>MKTENAKTNQTLVENSLNTQLSNWFLLYSKLHRFHWYVKGPHFFTLHEKFEELYDHAAETVD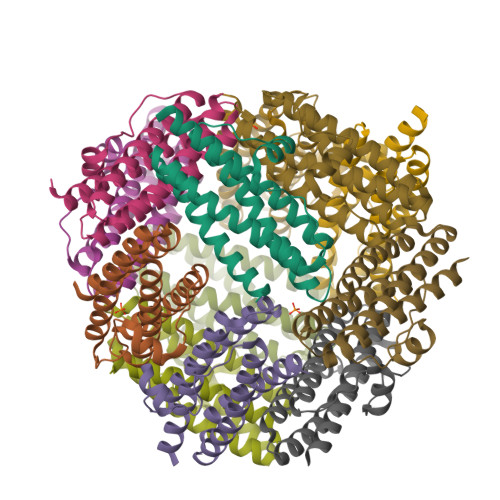TIAERLLAIGGQPVATVKEYTEHASITDGGNETSASEMVQALVNDYKQISSESKFVIGLAEENQDNATADLFVGLIEEVEKQVWMLSSYLG[4x]>[2x]MASMKFVTASYNVGYPAYGAKFLNNDTLLVAGGGGEGNNGIPNKLTVLRVDPTKDTEKEQFHILSEFALEDNDDS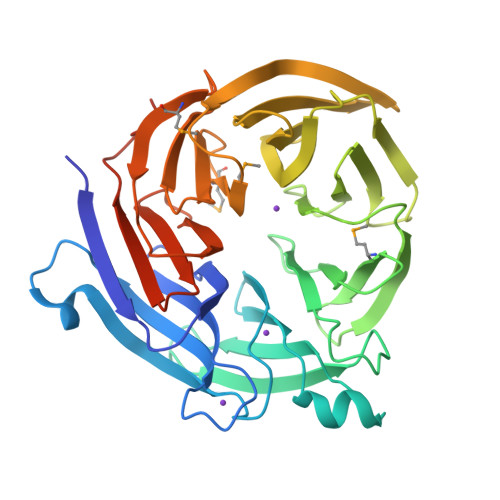PTAIDASKGIILVGCNENSTKITQGKGNKHLRKFKYDKVNDQLEFLTSVDFDASTNADDYTKLVYISREGTVAAIASSKVPAIMRIIDPSDLTEKFEIETRGEVKDLHFSTDGKVVAYITGSSLEVISTVTGSCIARKTDFDKNWSLSKINFIADDTVLIAASLKKGKGIVLTKISIKSGNTSVLRSKQVTNRFKGITSMDVDMKGELAVLASNDNSIALVKLKDLSMSKIFKQAHSFAITEVTISPDSTYVASVSAANTIHIIKLPLNYANYTSMKQKISKLEHHHHHH>[2x]MILDTDYITEDGKPVIRIFKKENGEFKIDYDRNFEPYIYALLKDDSAIEDVKKITAERHGTTVRVVRAEKVKKKFLGRPIEVWKLYFTHPQDQPAIRDKIKEHPAVVDIYEYDIPFAKRYLIDKGLIPMEGDEELKMLAFAIATLYHEGEEFAEGPILMISYADEEGARVITWKNIDLPYVDVVSTEKEMIKRFLKVVKEKDPDVLITYNGDNFDFAYLKKRSEKLGVKFILGREGSEPKIQRMGDRFAVEVKGRIHFDLYPVIRRTINLPTYTLEAVYEAIFGQPKEKVYAEEIAQAWETGEGLERVAR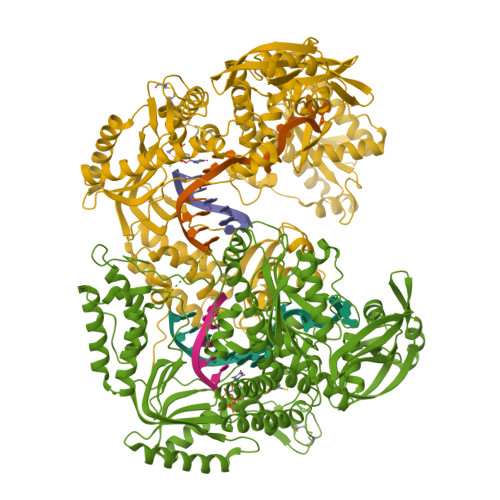YSMEDAKVTYELGKEFFPMEAQLSRLVGQSLWDVSRSSTGNLVEWFLLRKAYERNELAPNKPDERELARRRESYAGGYVKEPERGLWENIVYLDFRSLYPSIIITHNVSPDTLNREGCEEYDVAPQVGHKFCKDFPGFIPSLLGDLLEERQKVKKKMKATIDPIEKKLLDYRQRLIKILANSFYGYYGYAKARWYCKECAESVTAWGRQYIETTIREIEEKFGFKVLYADTDGFFATIPGADAETVKKKAKEFLDYINAKLPGLLELEYEGFYKRGFFATKKKYAVIDEEDKITTRGLKMVRRDWSEIAKETQARVLEAILKHGDVEEAVRIVKEVTEKLSKYEVPPEQLVIYQPITKQLHDYRARGPHVSVAKRLAARGIKIRPGTVISYIVPKGSGRIGDRAIPFDEFDPAKHKYDAGYYIENQVLPAVERILRAFGYRKEDLRYQKTRQVGLGAWLKPKT>[2x]MTATEELTFESTSRFAEVDVDGPLKLHYHEAGVGNDQTVVLLHGGGPGAASWTNFSRNIAVLARHFHVLAVDQPG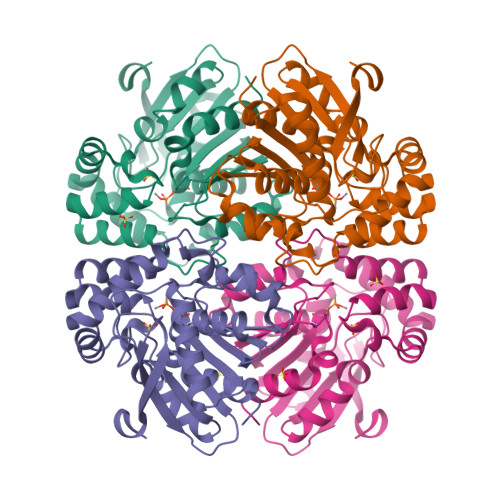YGHSDKRAEHGQFNRYAAMALKGLFDQLGLGRVPLVGNSLGGGTAVRFALDYPARAGRLVLMGPGGLSINLFAPDPTEGVKRLSKFSVAPTRENLEAFLRVMVYDKNLITPELVDQRFALASTPESLTATRAMGKSFAGADFEAGMMWREVYRLRQPVLLIWGREDRVNPLDGALVALKTIPRAQLHVFGQCGHWVQVEKFDEFNKLTIEFLGGGRKLHHHHHH~{N}-[2-methoxy-5-(phenylsulfamoyl)phenyl]-2-(4-oxidanylidene-3~{H}-phthalazin-1-yl)ethanamide | C23 H20 N4 O5 S | 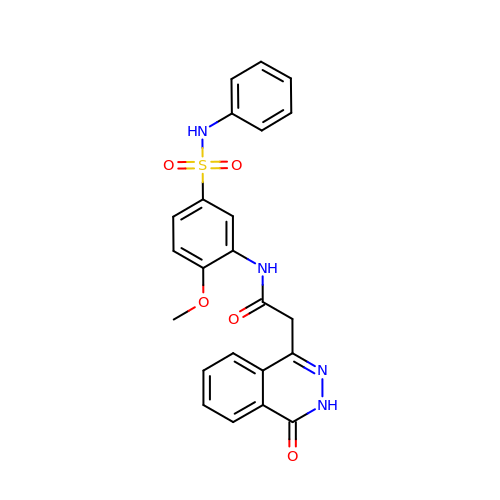XJTPZDXOGCHWMM-UHFFFAOYSA-N> ISAAAFDAAEQLIQVWDGTPEALVFEATEDEVAEYLSAVDVAIEHLARGSGGGAGGAGSSSSSTAGRAGVAVQLAMARLEEELRHLMVRHAVPLDPTGLFFSLRRLSLGSMDDLDTSSEFDAATPHSIDVAPETARGGPLVNPFEDQVFDPVRPEAVDDLRAIADRMARAGYSRELADAYCGIRRDLLDEYLSALGVERLSIDEVQRIEWKHLNDKMKKWVQAVKTVVRVLLAGERRLCDQVLSVSDELREECFIESTKGCIMQILSFGDAVAVCPRSPEKLSRILDMYEALAEVIPEMKDLCLGSSGDGVISDVQANLDRLGDAIRGTLFEFGKVLQLESSRRAMTAGEIHPMTRYVMNYLRLLVVYSDTLDALLDDNADDQIDLARAEDQDQEHLESMTPLGKRLLKLISYLEANLEEKSKLYEDSALECIFSMNNLLYIVQKVRDSELGKILGDHWVKRRNGKIRQYSKSYLRISWMKVLSFLKDDGHGSGSGSSSGSGSGHSSSRMSIKEKFKNFNLAFEEIYRNQTTWKVPDPQLREELKISISENVIPAYRAFLGRYGSQVDGGRNSGKYIKYTPEDLESQLSD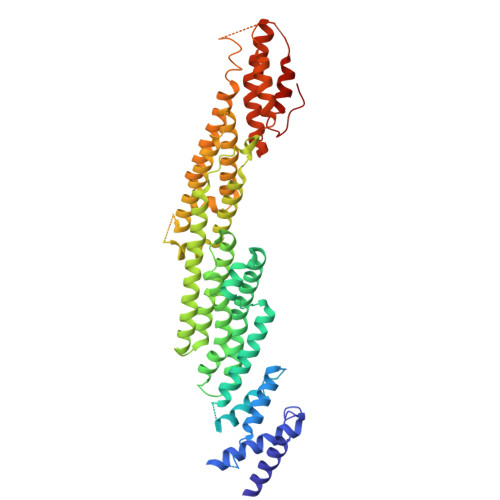LFEGAPGPANHSRRRT> GPLGSMEGEELIYHNIINEILVGYIKYYINDISEHELSPYQQQIKKILTYYDECLNKQVTITFSLTSVQEIKTQFTGVVTELFKDLINWGRICGFIVF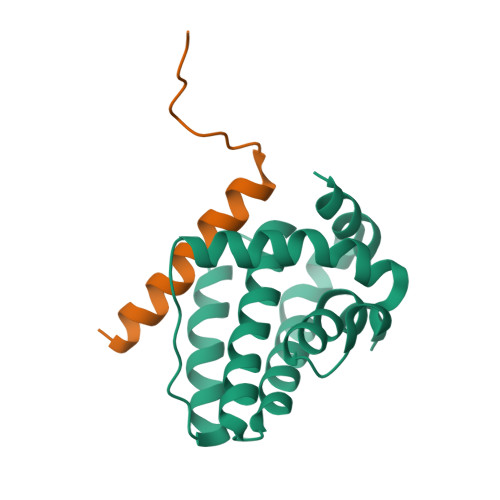SAKMAKYCKDANNHLESTVITTAYNFMKHNLLPWMISHGGQEEFLAFSLHSDMYS;> SESQEAVIRDIARHLARIGDRMEYGIRPGLVDSL> MSISASEARQRLFPLIEQVNTDHQPVRITSRAGDAVLMSADDYDAWQETVYLLRSPENARRLMEAVARDKAGHSAFTKSVDEL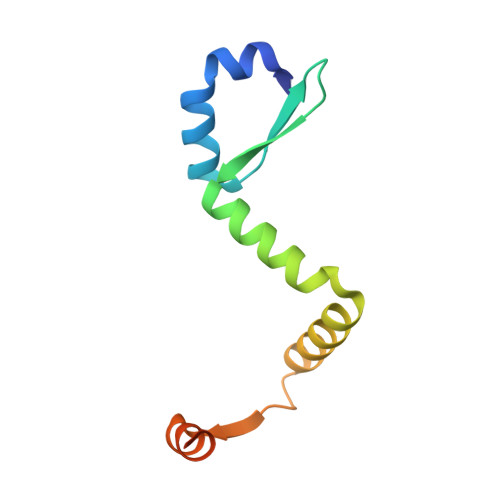REMAGGEEMQAGPAL> IAMPSVRKYAREKGVDIRLVQ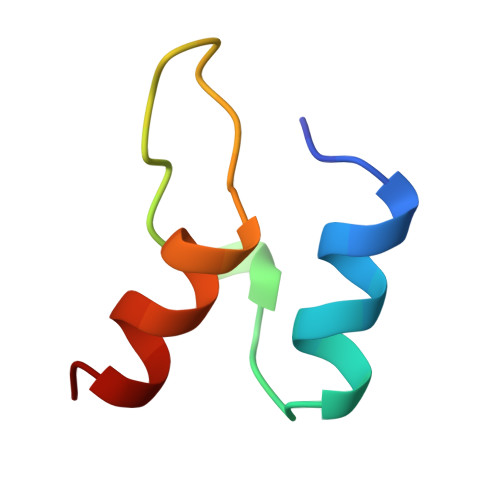GTGKNGRVLKEDIDAFLAGG1-(1~{H}-indol-3-yl)ethanone | C10 H9 N O | 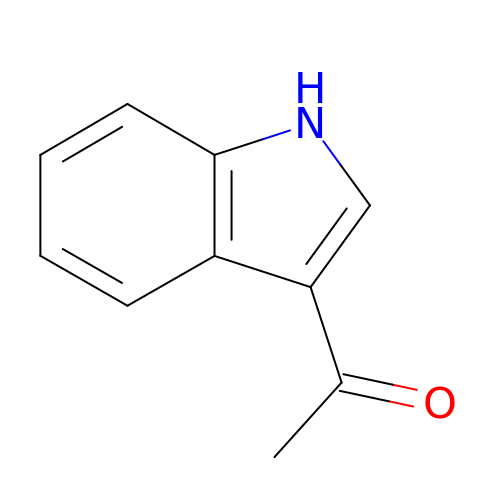VUIMBZIZZFSQEE-UHFFFAOYSA-N First, lipases are very versatile enzymes that catalyze the hydrolysis of ester linkages, primarily in neutral lipids such as triglycerides, which have been extensively characterized and used as CLECs in many studies and from different sources representing an excellent example of a biocatalyst and its applications. Finally, we determined the three-dimensional (3D) models of this commercial lipase crystallized with and without phosphate at 2.0 and 1.7 Å resolutions, respectively. In short, the structure of BioL corresponds to the typical α/β fold highly preserved among different species and has no difference in the catalytic triad composed by Ser146–His258–Asp201 with the nucleophilic Ser146, showing the strained conformation characteristic of the nucleophilic elbow. The structural model presents the closed state of the lid (residue 86–92), as present in many other structural models, which does not prevent the enzymatic activity in the crystals form as shown next.

Initial hits were obtained by the capillary counterdiffusion technique using 0.82 M K/NaH2PO4, 0.1 M Hepes, pH 7.5 (C23 of the CSK screening kit) or 5.0 M sodium formate in 100 mM AcNa pH 7.0 as precipitating agents. In a second step, we tested the compatibility of both conditions with the use of agarose (0.2% w/v) or silica (2.0% v/v) gels by loading the capillary with the mix of BioL and gels. For comparison purposes, we also determined the 3D structure of BioL obtained in the absence of phosphate from crystals grown in capillaries with sodium formate as a precipitant agent. Interestingly, these crystals also belong to the same space group, P61, but diffracted X-ray to a resolution of 1.7 Å, being the highest-resolution structures of TLL determined in the hexagonal space group and deposited in the PDB. Besides the great improvement on the resolution, when compared with the structure obtained using phosphate, chains A superimposed with an RMSD value of 0.34 and 0.49 Å when superimposing A and B chains at the same time using STAMP. The advantage of using a gel matrix media, e.g., agarose, is then exploited to: (i) produce homogeneous batches of crystals (500 mL), (ii) facilitate crystal stabilization by chemical cross-linking, and (iii) to obtain high-quality crystals (allowing to determine the three-dimensional (3D) model at 1.7 Å) and to facilitate crystal recovery.

>[2x]EVSQDLFNQFNLFAQYSAAAYCGKNNDAPAGTNITCTGNACPEVEKADATFLYSFEDSGVGDVTGFLALDNTNKLIVLSFRGSRSIENWIGNLNFDLKEINDICSGCRGHDGFTSSWRSVADTLRQKVEDAVREHPDYRVVFTGHSLGGALATVAGADLRGNGYDIDVFSYGAPRVGNRAFAEFLTVQTGGTLYRITHTNDIVPRLPPREFGYSHSSPEYWIKSGTLVPVTRNDIVKIEGIDATGGNNQPNIPDIPAHLWYFGLIGTCL> EVSAEEIKKHEEKWNKYYGVNAFNLPKELFSKVDEKDRQKYPYNTIGNVFVKGQTSATGVLIGKNTVLTNRHIAKFANGDPSKVSFRPSINTDDNGNTETPYGEYEVKEILQEPFGAGVDLALIRLKPDQNGVSLGDKISPAKIGTSNDLKDGDKLELIGYPFDHKVNQMHRSEIELTTLSRGLRYYGFTVPGNAGSGIFNSNGELVGIHSSKVSHLDREHQINYGVGIGNYVKRII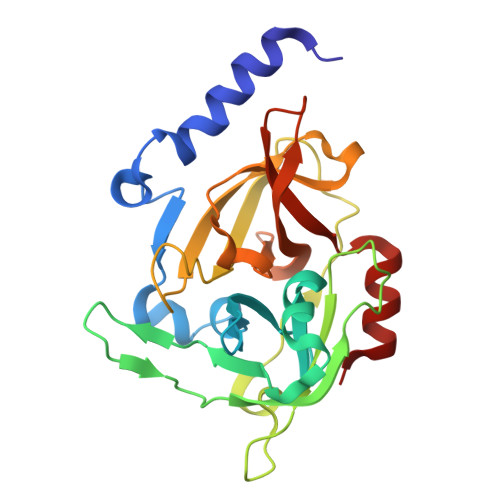NEKNE>SMDDSETGFNLKVVLVSFKQCLDEKEEVLLDPYIASWKGLVRFLNSLGTIFSFISKDVVSKLRIMERLRGGPQSEHYRSLQAMVAHELSNRLVDLERRSHHPESGCRTVLRLHRALHWLQLFLEGLRTSPEDARTSALCADSYN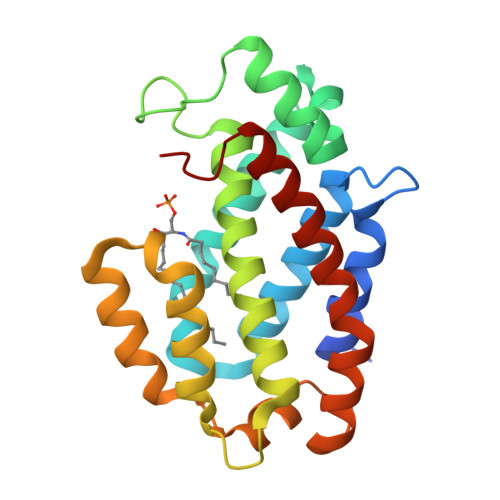ASLAAYHPWVVRRAVTVAFCTLPTREVFLEAMNVGPPEQAVQMLGEALPFIQRVYNVSQKLYAEHSLLDLP[4x]>[4x]SQPVAITDGIYWVGAVDWNIRYFHGPAFSTH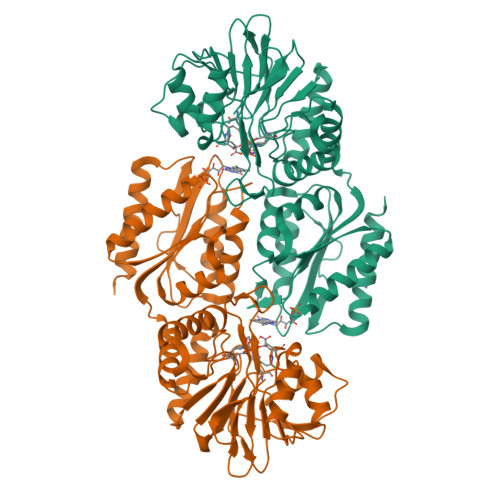RGTTYNAYLIVDDKTALVDTVYEPFKEELIAKLKQIKDPVKLDYLVVNHTESDHAGAFPAIMELCPDAHVLCTQRAFDSLKAHYSHIDFNYTIVKTGTSVSLGKRSLTFIEAPMLHWPDSMFTYVPEEALLLPNDAFGQHIATSVRFDDQVDAGLIMDEAAKYYANILMPFSNLITKKLDEIQKINLAIKTIAPSHGIIWRKDPGRIIEAYARWAEGQGKAKAVIAYDTMWLSTEKMAHALMDGLVAGGCEVKLFKLSVSDRNDVIKEILDARAVLVGSPTINNDILPVVSPLLDDLVGLRPKNKVGLAFGAYGWGGGAQKILEERLKAAKIELIAEPGPTVQWVPRGEDLQRCYELGRKIAARIAD>SNAVTDDLRLVDITETQLDDVLRVRARSFGLLAAGAREDWVRDAVEFVHDGRFLGVVSGDEVVAAARIWDFQQWWGGRRVPMAGIAGVVVAPEYRGRGVGSLLMRGVLERSRDKGMPISALYPATTVIYRHLGYEFGGHRYRFSFQAADLRSLGGREVAVRRAGAKDAARFLELVGTAHEASRASGLLVWPESKIAEWLEDEENFAYLAEDGFVVYNWSDGDLQVDELVAHSEATARALWATVGSGASIARTVHAYLSPNDPVHLLVEHEADKQAHVQRWMLRLLDAPAAIAARGFAPGAAAEVDLLID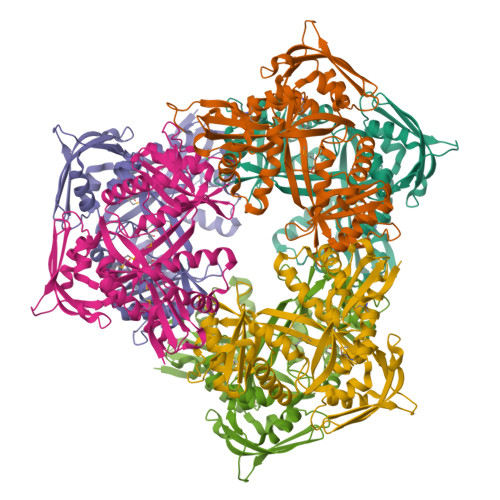DPGVPAQSGRWHLSVADGTGELTPSDRSGDVLQLGSRGLAALYAGTPLAALRTAGLVTGGPVASDRLLDTAFGGAAPYMLDYF[6x]> MASDVTVNLGSTKQEIRGFGASSAWCGTISDYVMNSLYGDLGYSILRLRIEEGIGDAWKTGNFSKWSPELANAKKASAKGAIVFASPWNPPASMQENFSKSGDSSAQRLRYDKYTEYAQYLNAYVKYMKDNGVDLYAISVQNEPDYAQDWTW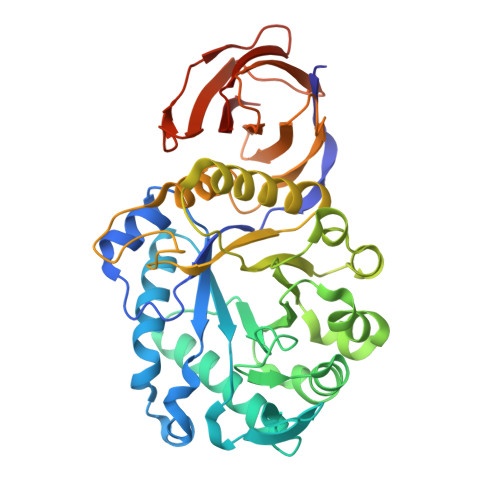WTPQEMLNFMKNNAGSINCRVMAPESFQFLKNMSDPILNDATALDNMDVLGCHFYGTSVNNMAYPLYQQKSAGKELWMTEKYFDDDTTGNIMNMSKEIHDSMVTGNMNAYIYWWITWPNGLATSSGTIYKRAYVLGQFAKFIRPGYKRVDATATPNTNVYVSAYTGDNKAVIVAINTGTAAVSQKFNFQNGSASSVVSYVTDSSRNMAAGANIAVTNGSFTAQLPAQSITTFVGNALEHHHHHH> MTDDKDVLRDVWFGRIPTCFTLYQDEITEREAEPYYLLLPRVSYLTLVTDKVKKHFQKVMRQEDISEIWFEYEGTPLKWHYPIGLLFDLLASSSALPWNI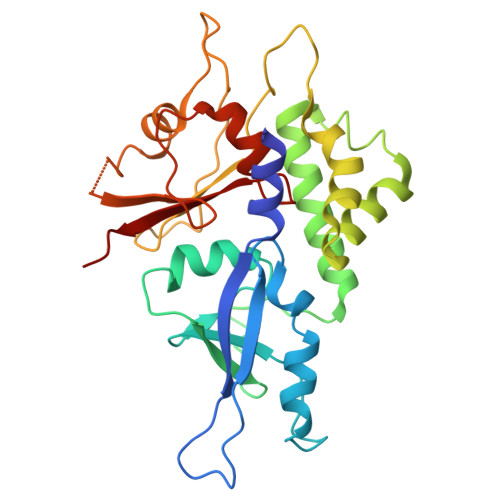TVHFKSFPEKDLLHCPSKDAIEAHFMSCMKEADALKHKSQVINEMQKKDHKQLWMGLQNDRFDQFWAINRKLMEYPAEENGFRYIPFRIYQTTTERPFIQKLFRPVAADGQLHTLGDLLKEVCPSAIDPEDGEKKNQVMIHGIEPMLETPLQWLSEHLSYPDNFLHISIIPQPTD>[2x]XLAAAAA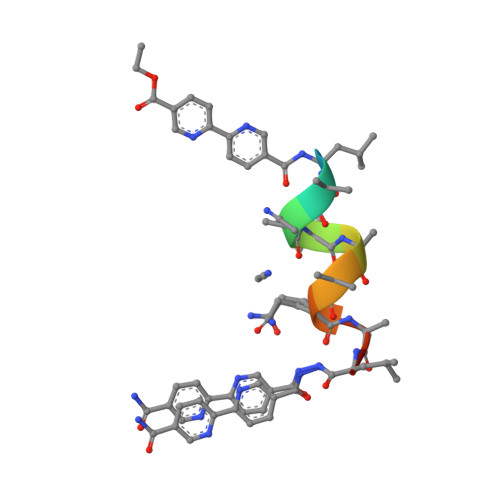QALX Three highly related Salmonella effectors, SseK1, SseK2, and SseK3, orthologues of the enteropathogenic and enterohemorrhagic Escherichia coli T3SS effector NleB1 (7), translocate via the T3SS into the host cell. Similarly to NleB1 (9, 10), SseK1 and SseK3 are N-acetylglucosamine (GlcNAc) transferases that modify the TNFR1-associated death domain protein TRADD and inhibit activation of the pro-inflammatory transcription factor NF-κB, as well as necroptotic host cell death. Here we report the structure of the Salmonella arginine N-glycosyltransferase, SseK3, in its apo and ligand-bound forms. The SseK3 catalytic core domain (∼250 residues) shows the classic features of the large glycosyltransferase type-A family of enzymes (GT-A) consisting of a single module composed of a central parallel β-sheet core flanked by a number of α-helices.

Crystals of SseK3(14–333) enriched with selenomethionine diffracted to good resolution, but most of them exhibited severe anisotropy, were non-isomorphous, and showed translational non-crystallographic symmetry. Attempts to solve the structure by molecular replacement using available glycosyltransferase X-ray structures or selenium SAD phasing failed. Instead, we recorded data at the I23 long-wavelength beamline at Diamond Light Source to reveal the positions of the selenium and sulfur atoms within SseK3 based on the small anomalous signals present at long wavelengths to obtain an initial model. This model was used as template in a molecular replacement search with a complete 2.21 Å resolution data set that did not exhibit severe diffraction anisotropy. that overlap with a root mean square deviation (RMSD) (Cα of residues 27–328) of 0.91 Å. The structure of apo-SseK3(14–333) is reported in Fig. 2A. Residues 14–25 are not visible in the electronic density for either chain, nor are amino acids 329–333 of chain B and the last serine residue (Ser-333) of chain A. Residues 27–321 of SseK3 in the apo and ligand-bound forms overlap with an RMSD of 0.84 Å, whereas residues 322–332 of SseK3(14–333) are unstructured with an average B factor of 45.5 Å2, compared with the average macromolecule B factor of 33.3 Å2. As suggested by solution NMR spectroscopy, the C-terminal residues are disordered in the unbound SseK3 structure, with structural reorganization following primary substrate binding, with an open-close catalytic cycle that, as in the case of a number of other glycosyltransferases, is likely to support SseK3 enzymatic activity. UDP-GlcNAc hydrolysis is not observed with SseK3(14–333) or in the absence of enzyme, indicating that together, the C-terminal residues Trp-334 and Arg-335 are necessary for SseK3 functional activity.

>GPLGSYSHTATPAITLPSSGSANFAGVEYPLLPLDQHTPLLFQWFERNPSRFGENQIPIINTQQNPYLNNIINAAIIEKERTIGVLVDGNFSAGQKKALAKLEKQYENIKVIYNSDLDYSMYDKKLSDIYLENIAKIEAQPANVRDEYLLGEIKKSLNEVLKNNPEESLVSSHDKRLGHVRFDFYRNLFLLKGSNAFLEAGKHGCHHLQPGGGCIYLDADMLLTGKLGTLYLPDGIAVHVSRKGNSMSLENGIIAVNRSEHPALKKGLEIMHSKPYGDPYIDGVCGGLRHYFNCSIRHNYEEFCNFIEFKHEHIFMDTSSLTISS[2x]>MNHKVHMITITGYSDVLSAGPGETVEFKVSSKSPHPFTAELVRVIHADPNPAGPGMRFEPLGQVFSGTFASFDKPLLPGSFARVSGVPAAGSAAGLVAGARIRPTALARGDQCVMSQWNTARHAGFALLVSERGLELRLGAGTGEPPVCVLCAARLEVRWYDVWFAIDTASNRIEVGVTEVDGSVAAPVRHRTLQMLDARWRAPHSDDAADLLIGALEDGAGRRAHFNGQIEAPFVADALPSPATPAATVEYAAPRASDFSTDALYAAWDFARGIDTLKIADTTPHARHGTLQNLPTRAVRSSAWNGRERCWRTAPAHYAAIHFHDDDLHDAGWSTDFAFTVPATLKSGAYAMRLSVDGATDYLPFYVRPELGRPGAPLVFVAATYTYQAYANYARGNFDAALRDKVGRWGAYPHNPDDHPEVGLATYNLHSDGSGVMFSSRLRPMLTMRPGFLTFDDSRGSGCRHYIADSHLLDWLEHEGFSFDVVTDDDLERFGAALLEPYAAVLTGTHPEYHTAATLDALAGYKRSGGNLAYLGGNGFYWRVGRSERVPGALEVRRTEGGVRAWAAEAGEYFHALDGEYGGLWRSSARTPQQLVGVGFSSQGPFEGSHYRVLDA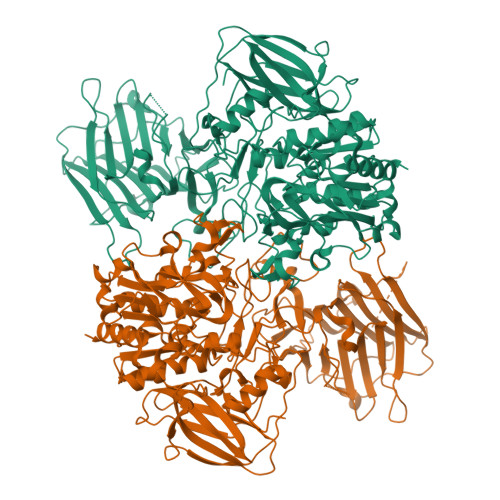ARSQPGGSLLKDIAGPLFGGYGLSGGGAAGFELDSTEAADGTPANVIILARSESHSAAFGPALDALLSHTATRARKTPDTLIRSEIVYYETGYGGAVFSVGSITFCGALSHNDYRNDVSTLLRNVLIRFSRDRGAQAHAVPAVAHTEVDHHHHHH[2x]>[2x]MGELRVGLEESELWLRFKELTNEMIVTKNGRRMFPVLKVNVSGLDPNAMYSFLLDFVAADNHRWKYVNGEWVPGGKPEPQA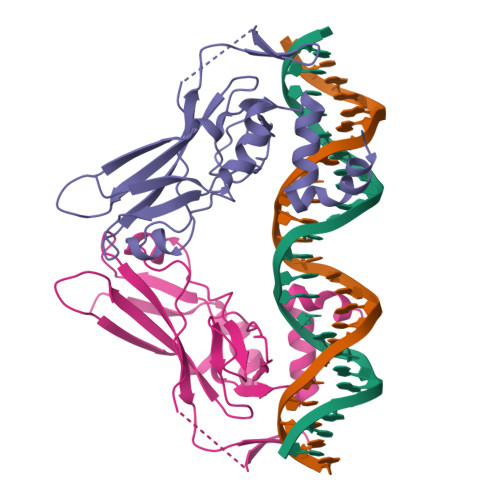PSCVYIHPDSPNFGAHWMKAPVSFSKVKLTNKLNGGGQIMLNSLHKYEPRIHIVRVGGPQRMITSHCFPETQFIAVTAYQNEEITALKIKYNPFAKAFLDAKERSHHHHHH>SNADTSKEKGGSKETVPEKNLDSFTLSGYIYTYENAPQEIRDEHKQNCEEINIDPKPDDEIFVPESANLMNEDNSKGVYASYTVSYNIGAKTITIMSNEYLTISTTKVIRKGNSGKEVKAAQIMLTLLGYNVGIDSSFGSKTYNAVVSFQKK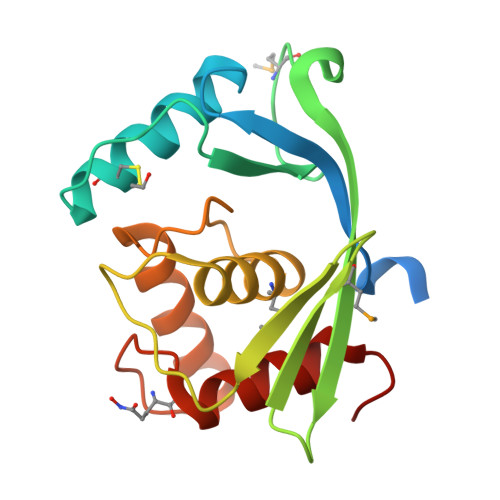YGLSADGIIGPATWDKLGRLTDPTLS[2x]> MDRRKFIKTSLFSALGFSVGGLSLLSCGGGGTTGSSSGQGSGTLSKQSLNIPGYFLFPDGQRVSITAKWTTLEVIPGKSTDMLVYEIDNEYNPVIFLRKGQTFSADFVNNSGEDSIIHWHGFRAPWKSDGHPYYAVKDGETYSYPDFTIIDRSGTYFYHPHPHGRTGYQVYYGLAGMIIIEDEDEDNLKQALDLEYGVIDIPLIIQDKTFDSSGQLVYNPMGHMGFWGDTILVNLTPNPYMDVERKIYRFRILNGSNARPYRLALLRGNQRMRFWVIGVEGGLLDTPKEVNEILVAPGERIDILVDFRDASVNDVIKLYNFPHNLIGMGMIGMRMGM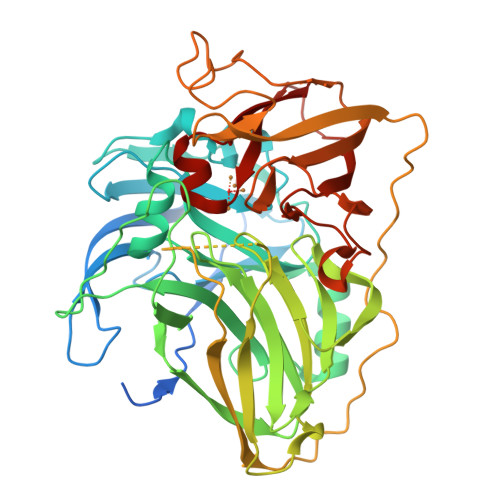GMERGMGMGNGMNMDMGMADNSEFEVMEFRVTKDSAYDKSIPQRLSEVTPINTDGAQVQRITLGMRRMVFTINGETWEDGYANPQDINNPKVLFEQNNGDVVIIEYVNNTGMYHPMHIHGFQFQVLERSLGPLRATDLGWKDTVIVAPMETVRIAVDMSHPYNEHQIYLLHCHILEHHDEGMMVNYRVNA>DAASHEE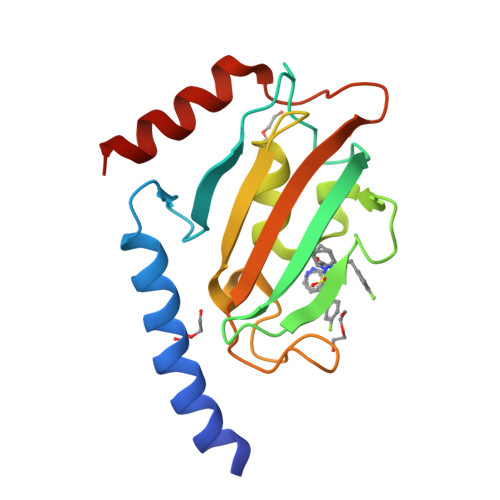RMNNYRKRVGRLFMEQKAAQPDAVKLPSGLVFQRIARGSGKRAPAIDDKCEVHYTGRLRDGTVFDSSRERGKPTTFRPNEVIKGWTEALQLMREGDRWRLFIPYDLAYGVTGGGGMIPPYSPLEFDVELISIKDGGKGRTAEEVDEILRKAEED[2x]(2S)-N~1~-benzyl-2-[(4-fluorophenyl)methyl]-N~3~-hydroxypropanediamide 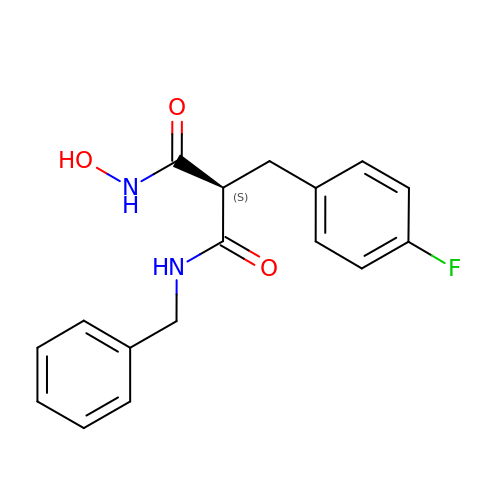| C17 H17 F N2 O3 | UBULRDFJXZRBJH-HNNXBMFYSA-N L‐Asparaginases (ASNases) catalyze the hydrolysis of L‐Asn to L‐Asp and ammonia. In contrast, the chain of ASNase from Rhodospirillum rubrum, reported here and referred to as RrA, consists of only 172 amino acid residues. RrA is homologous to the N‐terminal domain of typical bacterial class 1 ASNases and exhibits millimolar affinity for L‐Asn. Crystal structures of the wild‐type RrA, both with and without bound L‐Asp, as well as structures of several RrA mutants, reveal topologically unique tetramers.

Mutation of Lys158 was anticipated to impede the completion of the catalytic event by preventing the second step of the reaction that would result in hydrolysis of the covalent acyl‐enzyme intermediate (Lubkowski et al., 2020). RrA(K168M) was crystallized in the presence of L‐Asp. However, the density present in the active site could be modeled only by several water molecules. The methionine side chains in the mutated site were modeled with two orientations of unequal occupancy. A water molecule forms a bridge between Lys19 and Thr16 of one protomer, as well as with Tyr21 of another protomer. Similar to the situation found in typical class 1 ASNases, mutation of the catalytic Lys residue (K158M in RrA) completely inactivates the enzyme (Lubkowski et al., 2020; Strzelczyk et al., 2020; Strzelczyk et al., 2023).

>[2x]HHHHHHENLYFQSMAVSPSPLRIFTAGGTIDKDYRLEENGLVVGDPFVAEVLKTARLAGAVSIVALSRKDSLDFTEADREAIGRAVGQAVEDHILLTHGTDTMVETARYLGGLPELAGKTVVLSGAMVPGRVGGSDAAFNIGFACAAALMLAPGVYIAMHGKVFDPAKTRMNRGLGRFEPIDDQE>VHHPPSYVAHLASDFGVRVFQQVAQASKDRNVVFSPYGVASVLAMLQLTTGGETQQQIQAAMGFKIDDKGMAPALRHLYKELMGPWNKDEISTTDAIFVQRDLKLVQGFMPHFFRLFRSTVKQVDFSEVERARFIINDWVKTHTKGMISHLLGTGAVDQLTRLVLVNALYFNGQWKTPFPDSSTHRRLFHKSDGSTVSVPMMAQTNKFNYTEFTTPDGHYYDILELPYHGDTLSMFIAAPYEKEVPLSALTNILSAQLISHWKGNMTRLPR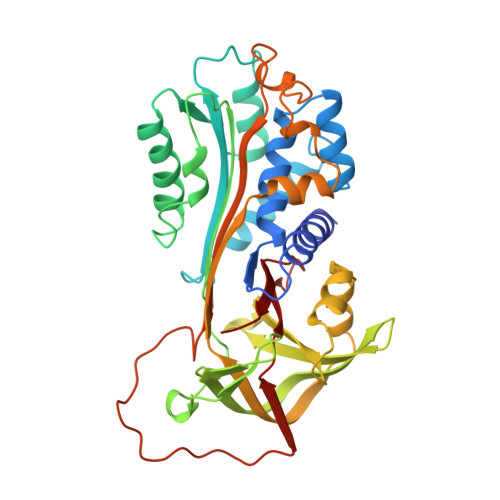LLVLPKFSLETEVDLRKPLENLGMTDMFRQFQADFTSLSDQEPLHVALALQKVKIEVNESGTVASSSTAVIVSARMAPEEIIIDRPFLFVVRHNPTGTVLFMGQVMEP[4x]>SGISLDNSYKMDYPEMGLCIIINNKNFHKSTGMTSRSGTDVDAANLRETFR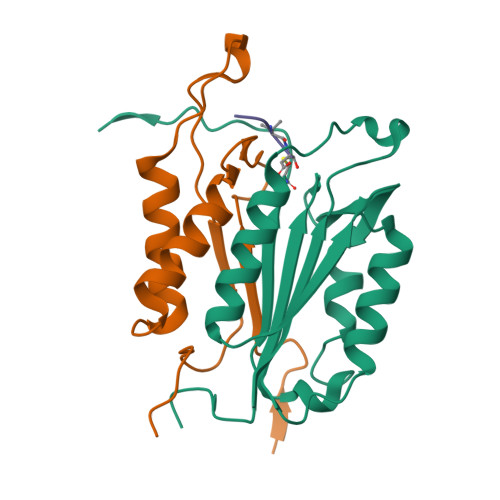NLKYEVRNKNDLTREEIVELMRDVSKEDHSKRSSFVCVLLSHGEEGIIFGTNGPVDLKKITNFFRGDRCRSLTGKPKLFIIQACRGTEYDCGIETD[2x];>[2x]SGVDDDMACHKIPVEADFLYAYSTAPGYYSWRNSKDGSWFIQSLCAMLKQYADKLEFMHILTRVNRKVATEFESFSFDATFHAKKQIPCIVSMLTKELYFYHHHHHHH> MSLRPCFVSLIDESDKPILIYVPNEAENEMNDVLKYNVLSNISLDYFESALVEWHSLDSKPLLKSIF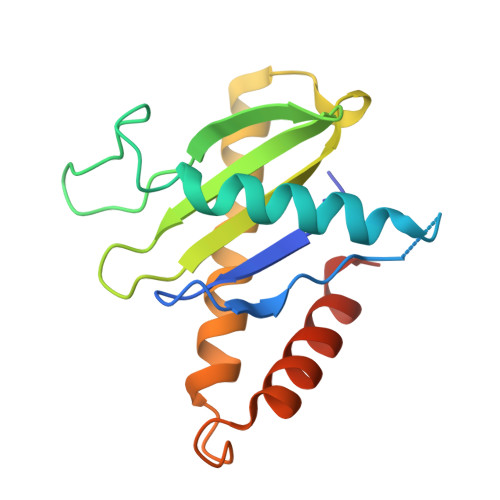QLEGVSVFAMLIKQTGLKIVIGFEQKSLSGADDEFEAINQIFETVRKIYIRVKCNPLLVSGDEKSIIKSLERKFDELFISTEVEL>[2x]MGGHHHHHHGENLYFQGISSETGEMGILWEFDPIINKWIRLSMKLKVERK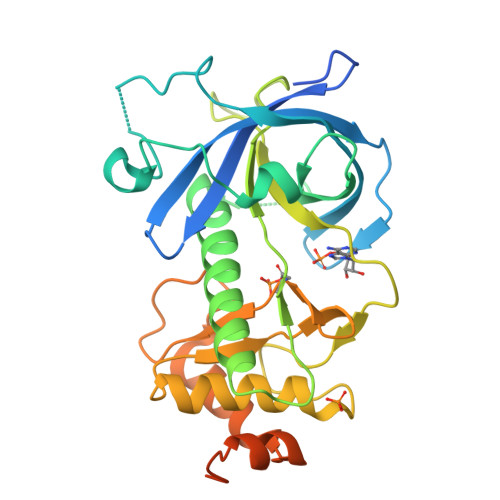PFAEGALREAYHTVSLGVGTDENYPLGTTTKLFPPIEMISPISKNNEAMTQLKNGTKFVLKLYKKEAEQQASRELYFEDVKMQMVCRDWGNKFNQKKPPKKIEFLMSWVVELIDRSPSSNGQPILCSIEPLLVGEFKKNNSNYGAVLTNRSTPQAFSHFTYELSNKQMIVVDIQGVDDLYTDPQIHTPDGKGFGLGNLGKAGINKFITTHKCNAVCALLDLDVKLGGVLSGNNKKQLQQGTMVMPDILPELMPSDNT>[3x]MLAKRIIACLDVKDGRVVKGTNFENLRDSGDPVELGKFYSEIGIDELVFLDITASVEKRKTMLELVEKVAEQIDIPFTVGGGIHDFETASELILRGADKVSINTAAVENPSLITQIAQTFGSQAVVVAIDAKRVDGEFMVFTYSGKKNTGILL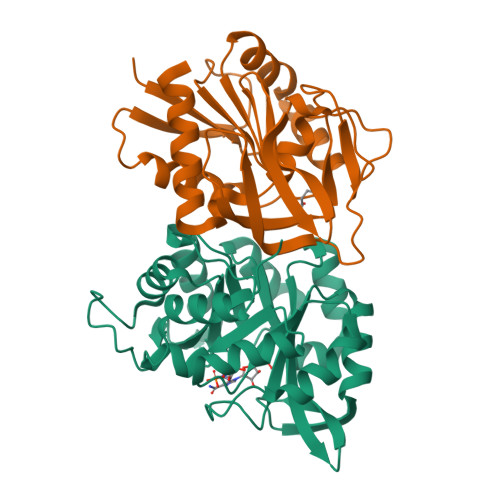RDWVVEVEKRGAGEILLTSIDRDGTKSGYDTEMIRFVRPLTTLPIIASGGAGKMEHFLEAFLAGADAALAASVFHFREIDVRELKEYLKKHGVNVRLEGL;>[3x]MGMRIGIISVGPGNIMNLYRGVKRASENFEDVSIELVESPRNDLYDLLFIPGVGHFGEGMRRLRENDLIDFVRKHVEDERYVVGVALGMQLLFEESEEAPGVKGLSLIEGNVVKLRSRRLPHMGWNEVIFKDTFPNGYYYFVHTYRAVCEEEHVLGTTEYDGEIFPSAVRKGRILGFQFHPEKSSKIGRKLLEKVIECSLSRR>[8x]GHMNHKDWDFVNRQLVAKMLAELEYEQVFHAESQGDGRYCINLPGAQWRFSAERGIWGWLWIDAQTLRCADEPVLAQTLLMQLKPVLSMSDATVAEHMQDLYATLLGDLQLLKARRGLSASDLIDLDADRLQCLLSGHPKFAFNKGRRGWGKEALERYAPEYANTFRLHWLAVKREHMVWRCDGSLTIGTLLAAAMDPQEFARFNQVWQDNGLDNDWLPLPVHPWQWQQKISLDFIADLAEGRMVSLGEFGDLWLAQQSLRTLTNASRQGGLDIKLPLTIYNTSCYRGIPGKYIAAGPLASRWLQQVFATDATLKQSGAVILGEPAAGYVSHEGYAAL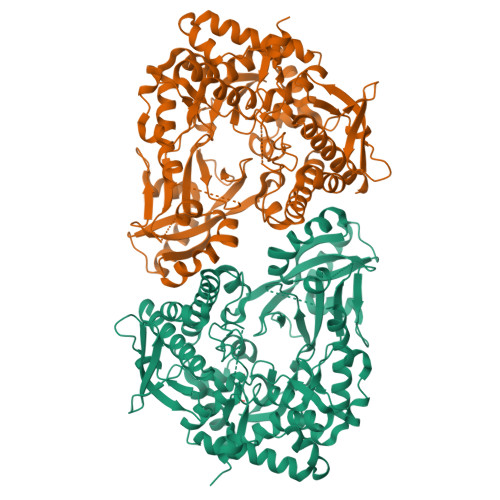AQAPYRYQEMLGVIWRENPCRWLKPDESPILMATLMECDENNQPLIGAYIDRSGLDAETWLTQLFRVVVVPLYHLLCRYGVALIAHGQNITLAMKKGVPQRVLLKDFQGDMRLVKDAFPEMDSLPQEVRDVTARLSADYLIHDLQTGHFVTVLRFVSPLMARLGVPERRFYQLLAAVLSDYMQEHPQMSARFALFSLFKPQIIRVVLNPVKLTWHDQDGGSRMLPNYLEDLQNPLWLATRD>DSNGNQEINGKEKLSVNDSKLKDFGKTVPVGIDEENGMIKVSFMLTQQFYEIKPTKENEQYIGMLRQAVKNESPVHIFLKPNSNEIGKVESASPEDVRYFKTILTKEVKGQTNKLASVIPDVATLNSLFNQIKNQSCGTSTASSPCITFRYPVDGCYARAHKMRQILMNNGYDCEKQFVYGNLKASTGTCCVAWSYHVAILVSYKNASGVTEKRIIDPSLFSSGPVTDTAWRNACVNTSCGSASVSSYANTAGNVYYRSPSNSYLYDNNLINTNCVLTKFSLLSGCSPSPAP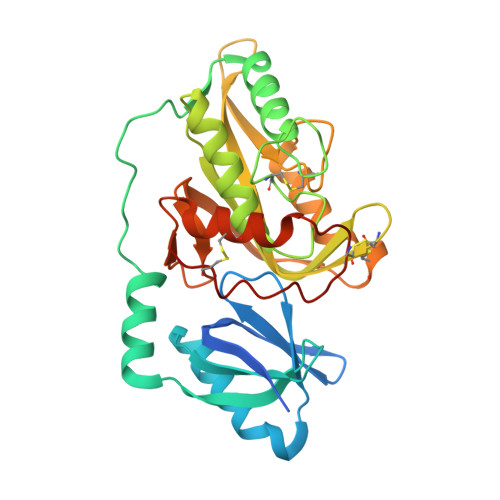DVSSCGFHHHHHH[2x]> GSDELYRQSLEIISRYLREQATGAKD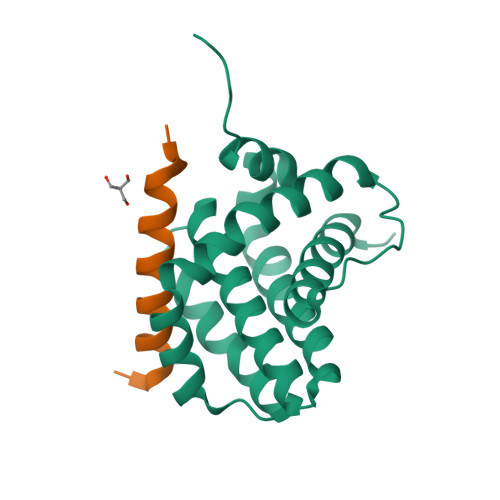TKPMGRSGATSRKALETLRRVGDGVQRNHETAFQGMLRKLDIKNEDDVKSLSRVMIHVFSDGVTNWGRIVTLISFGAFVAKHLKTINQESCIEPLAESITDVLVRTKRDWLVKQRGWDGFVEFFHVEDLEGG;> GSGGRPEIWYAQELRRIGDEFNAYYAR> MTWLPFIIIIPLLGAFSMPIVSLLKGKAKEIWASMISFATLIVGIQVFREVWSKGTIVYTLGAPNPFGKATFPIRIVWEVDKFGALMVLIVTFVSFLAVIYSIEYMKHDTGLEKFYTLILILELGMLGIAITGDIFNFYV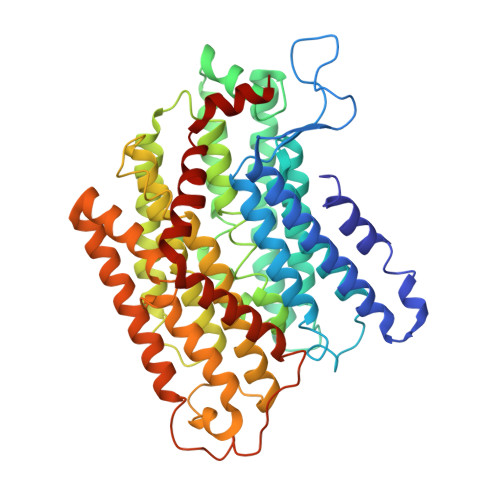FLEIMSIASYALVAFRNDTWEGIEAGIKYMFAGSLASSFVLLGIALLYGQYGTLTMGYLAVKIAENPTIVAKVALALFIGGLLFKSGAAPVHMWLADAHPAAPSSISAMLSGLVIKIGGIYAIARIVFSIFSPTINLGTIGWIIIIFACITLIVGNAMAVVQEDLKRLLAYSSVGQIGYILLGLGIGMVAYGTRVGEIALAGAIYHTVNHALMKALLFLVAGAVIHEIGTRNMNELSGLAKTMPKTTFAFLIGAAAIVGLPPLNGFASKWLIYESSALFNPILGAIAVIGTVFCTAAYVRALFTFFGRPSEKVTNARDPGIAMMLPMIILVVTIIVMGFFPWQISDRIMVPTARALWDVIDYISSLMGGG> RATPRMEDLASTDLSTRATGSINAVYFTNWGIYGRNFQPADLQASKILHVLYSFMNLRVDGTVYSGDTYADLEKHYSDDSWNDIGTNAYGCVKQLYKLKKANRSLKIMLSIGGWTWSTNFPAAASTEATRATFAKTAVEF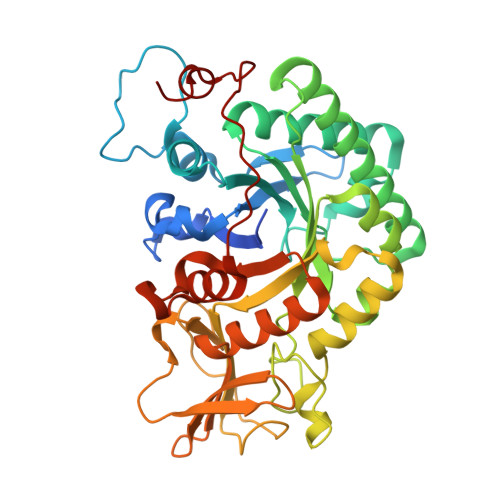MKDWGFDGIDVDWEYPASETDANNMVLLLQRVRQELDSYSATYANGYHFQLSIAAPAGPSHYNVLKLAQLGSVLDNINLMAYDYAGSWDSVSGHQTNLYPSTSNPSSTPFSTKAAVDAYIAAGVPASKIILGMPIYGRAFVGTDGPGKPYSTIGEGSWESGIWDYKVLPKAGATVITDSAAGATYSYDSSSRTMISYDTPDMVRTKVSYAKGLGLGGSMFWEASADKTGSDSLIGTALSSMGSHDSTQNCLSYPNSKFDNIKNSLS> MESEMLQSPLLGLGEEDEADLTDWNLPLAFMKKRHCEKIEGSKSLAQSWRMKDRMKTVSVALVLCLNVGVDPPDVVKTTPCARLECWIDPLSMGPQKALETIGANLQKQYENWQPRARYKQSLDPTVDEVKKLCTSLRRNAKEERVLFHYNGHGVPRPTVNGEVWVFNKNYTQYIPLSIYDLQTWMGSPSIFVYDCSNAGLIVKSFKQFALQREQELEVAAINPNHPLAQMPLPPSMKNCIQLAACEATELLPMIPDLPADLFTSCLTTPIKIALRWFCMQKCVSLVPGVTLDLIEKIPGRLNDRRTPLGELNWIFTAITDTIAWNVLPRDLFQKLFRQDLLVASLFRNFLLAERIMRSYNCTPVSSPRLPPTYMHAMWQAWDLAVDICLSQLPTIIEEGTAFRHSPFFAEQLTAFQVWLTMGVENRNPPEQLPIVLQVLLSQVHRLRALDLLGRFLDLGPWAVSLALSVGIFPYVLKLLQSSARELRPLLVFIWAKILAVDSSCQADLVKDNGHKYFLSVLADPYMPAEHRTMTAFILAVIVNSYHTGQEACLQGNLIAICLEQLNDPHPLLRQWVAICLGRIWQNFDSARWCGVRDSAHEKLYSLLSDPIPEVRCAAVFALGTFVGNSAERTDHSTTIDHNVAMMLAQLVSDGSP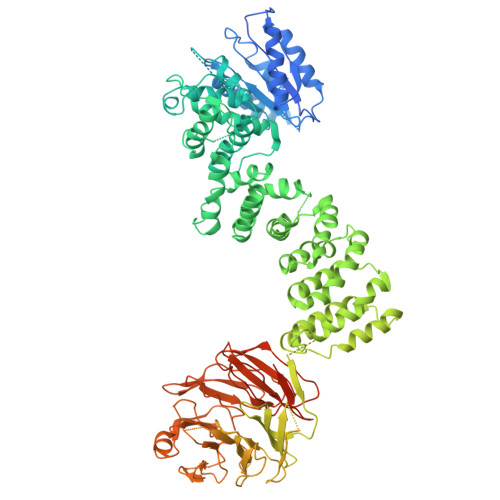MVRKELVVALSHLVVQYESNFCTVALQFIEEEKNYALPSPATTEGGSLTPVRDSPCTPRLRSVSSYGNIRAVATARSLNKSLQNLSLTEESGGAVAFSPGNLSTSSSASSTLGSPENEEHILSFETIDKMRRASSYSSLNSLIGVSFNSVYTQIWRVLLHLAADPYPEVSDVAMKVLNSIAYKATVNARPQRVLDTSSLTQSAPASPTNKGVHIHQAGGSPPASSTSSSSLTNDVAKQPVSRDLPSGRPGTTGPAGAQYTPHSHQFPRTRKMFDKGPEQTADDADDAAGHKSFISATVQTGFCDWSARYFAQPVMKIPEEHDLESQIRKEREWRFLRNSRVRRQAQQVIQKGITRLDDQIFLNRNPGVPSVVKFHPFTPCIAVADKDSICFWDWEKGEKLDYFHNGNPRYTRVTAMEYLNGQDCSLLLTATDDGAIRVWKNFADLEKNPEMVTAWQGLSDMLPTTRGAGMVVDWEQETGLLMSSGDVRIVRIWDTDREMKVQDIPTGADSCVTSLSCDSHRSLIVAGLGDGSIRVYDRRMALSECRVMTYREHTAWVVKASLQKRPDGHIVSVSVNGDVRIFDPRMPESVNVLQIVKGLTALDIHPQADLIACGSVNQFTAIYNSSGELINNIKYYDGFMGQRVGAISCLAFHPHWPHLAVGSNDYYISVYSVEKRVR> IKGGLFADIASHPWQAAIFAKHRRSPGERFLCGGILISSCWILSAAHCFQERFPPHHLTVILGRTYRVVPGEEEQKFEVEKYIVHKEFDDDTYDNDIALLQLKSDSSRCAQESSVVRTVALPPADLQLPDWTECELSGYGKHEALSPEYSERLKEAHVR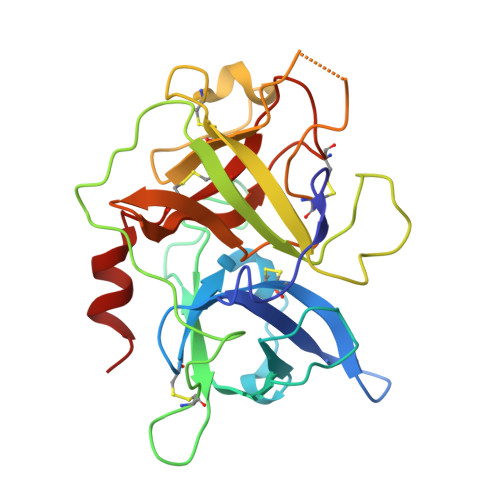LYPSSRCTSQHLLQRTVTDNMLCAGDTRSGGPQANLHDACQGDAGGPLVCLNDGRMTLVGIISWGLGCGQKDVPGVYTKVTNYLDWIRDNMR>MNPESRVIRKVLALQNDEKIFSGERRVLIAFSGGVDSVVLTDVLLKLKNYFSLKEVALAHFNHMLRESAERDEEFCKEFAKERNMKIFVGKEDVRAFAKENRMSLEEAGRFLRYKFLKEILESEGFDCIATAHHLNDLLETSLLFFTRGTGLDGLIGFLPKEEVIRRPLYYVKRSEIEEYAKFKGLRWVEDETNYEVSIPRNRIRHRVIPELKRINENLEDTFLKMVKVLRAEREFLEEEAQKLYKEVKKGNCLDVKKLKEK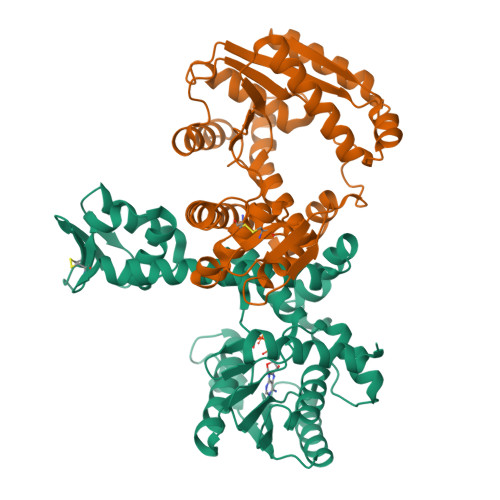PLALQRRVIRKFIGEKDYEKVELVRSLLEKGGEVNLGKGKVLKRKERWLCFSPEV[4x]>MEVVHFLEGVCFEKLHIEVLNENSSHKEIRIC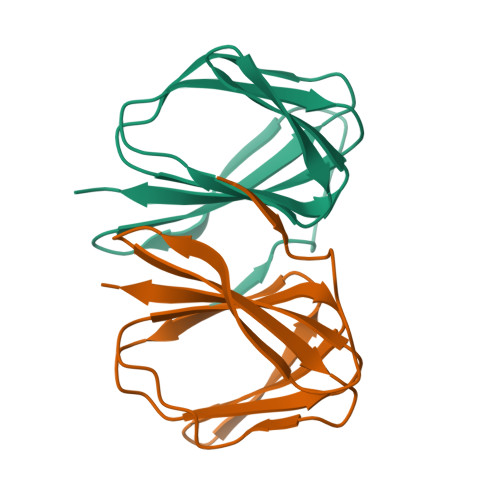MPKGAVMDKHKAPGAISVQVLEGKIVFEVGDEKIEMPKGALISLEAQVLHRLDALENSVIRLSLSKKLEHHHHHH[2x]4-oxidanylbutyl ~{N}-[4-[(4-aminophenyl)methyl]phenyl]carbamate | C18 H22 N2 O3 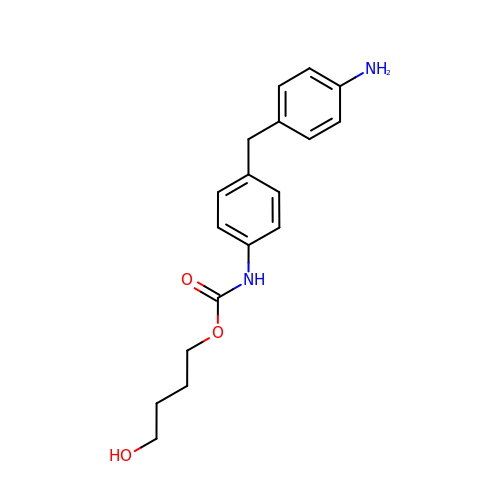| UWOCPQGJYMGPEI-UHFFFAOYSA-N>[2x]GFKQDIATIRGDLRTYAQDIFLAFLNKYPDERRYFKNYVGKSDQELKSMAKFGDHTEKVFNLMMEVADRATDSVPLASDANT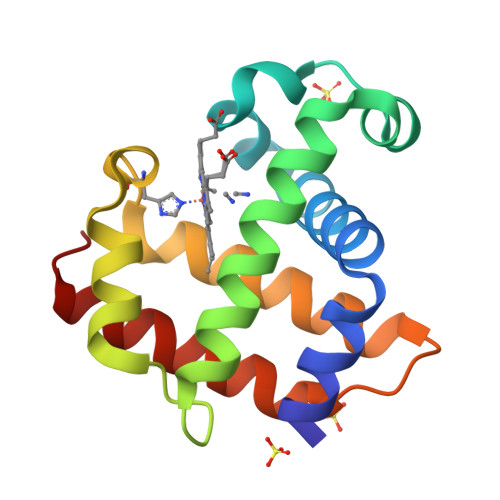LVQMKQHSSLTTGNFEKLFVALVEYMRASGQSFDSQSWDRFGKNLVSALSSAGMK> MKEFYLTVEQIGDSIFERYIDSNGRERTREVEYKPSLFAHCPESQATKYFDIYGKPCTRKLFANMRDASQWIKRMEDIGLEALGMDDFKLAYLSDTYNYEIKYDHTKIRVANFDIEVTSPDGFPEPSQAKHPIDAITHYDSIDDRFYVFDLLNSPYGNVEEWSIEIAAKLQEQGGDEVPS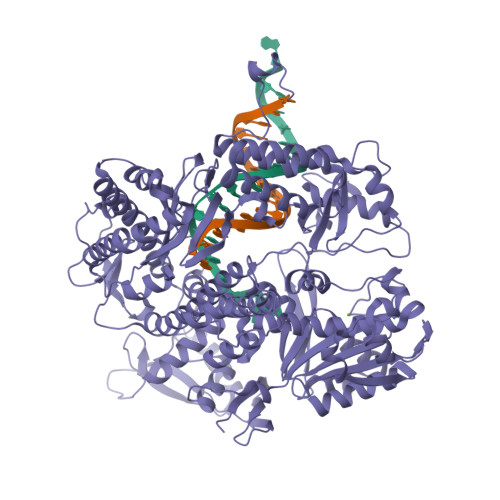EIIDKIIYMPFDNEKELLMEYLNFWQQKTPVILTGWNVESFAIPYVYNRIKNIFGESTAKRLSPHRKTRVKVIENMYGSREIITLFGISVLDYIDLYKKFSFTNQPSYSLDYISEFELNVGKLKYDGPISKLRESNHQRYISYNIIDVYRVLQIDAKRQFINLSLDMGYYAKIQIQSVFSPIKTWDAIIFNSLKEQNKVIPQGRSHPVQPYPGAFVKEPIPNRYKYVMSFDLTSLYPSIIRQVNISPETIAGTFKVAPLHDYINAVAERPSDVYSCSPNGMMYYKDRDGVVPTEITKWVSQRKEHKGYMLAAQRNGEIIKEALHNPNLSVDEPLDVDYRFDFSDEIKEKIKKLSAKSLNEMLFRAQRTEVAGMTAQMALKVTCNSLYGALGNVWFRYYDLRNATAITTFGQMALQWIERKVNEYLNEVCGTEGEAFVLYGDTDSIYVSADKIIDKVGESKFRDTNHWVDFLDKFARERMEPAIDRGFREMCEYMNNKQHLMFMDREAIAGPPLGSKGIGGFWTGKKRYALNVWDMEGTRYAEPKLKIMGLETQKSSTPKAVQKALKECIRRMLQEGEESLQEYFKEFEKEFRQLNYISIASVSSANNIAKYDVGGFPGPKCPFHIRGILTYNRAIKGNIDAPQVVEGEKVYVLPLREGNPFGDKCIAWPSGTEITDLIKDDVLHWMDYTVLLEKTFIKPLEGFTSAAKLDYEKKASLFDMFDFSAWSHPQFEK> NSSKSLEAELVRDRQELIDARKKELKAYMMMGVTAIKPLYDSDVNGSNKQAAKEILKAMRFESDGYFFAYDSQGINTLHAIKPSLEGKNLYDLKDENGVAVIAGLIDASQKGDGFLYFSWHKPTINAQAPKLGYAEYLQKWDWVLGTGIYIDDIDQQVAMQRELRTQELNQHT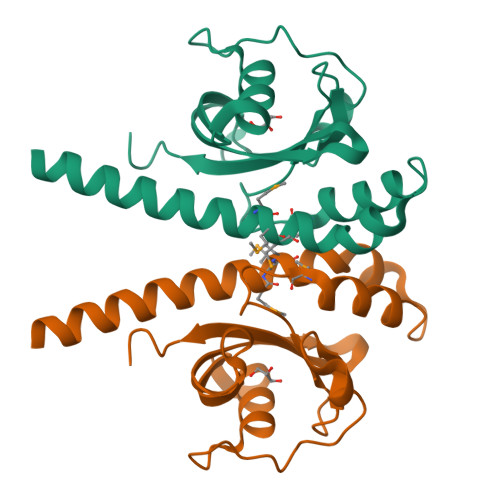I> RRLRAERWKAENQEGMAEVARFIEMNGSFADENRD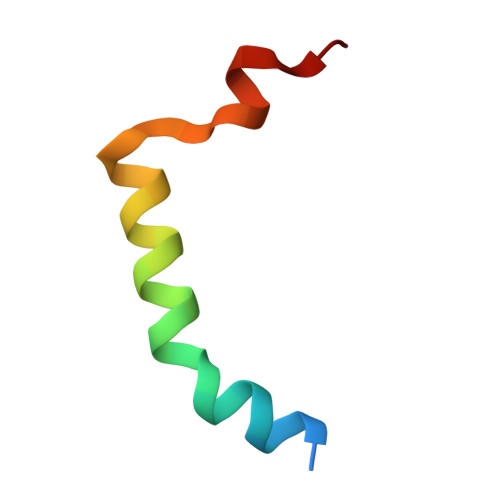W> QDADKLPHTKVTLVAPPQVHPHEQATKSGPKVVEFTMTIEEKKMVIDDKGTTLQAMTFNGSMPGPTLVVHEGDYVQLTLVNPATNAMPHNVDFHGATGALGGAKLTNVNPGEQATLRFKADRSGTFVYHAAPEGMVPWHVVSGMSGTLMVLPRDGLKDPQGKPLHYDRAYTIGEFDLYIPKGPDGKYKDYATLAESYGDTVQVMRTLTPSHIVFNGKVGALTGANALTAKVGETVLLIHSQANRDTRPHLIGGHGDWVWETGKFANPPQRDLETWFIRGGSAGAALYTFKQPGVYAYLN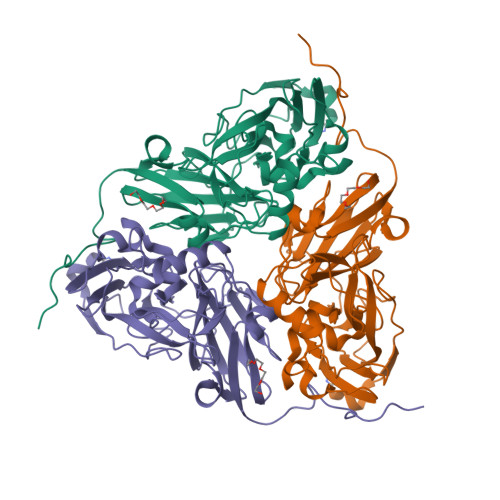HNLIEAFELGAAGHIKVEGKWNDDLMKQIKAPAPIPR> SDKII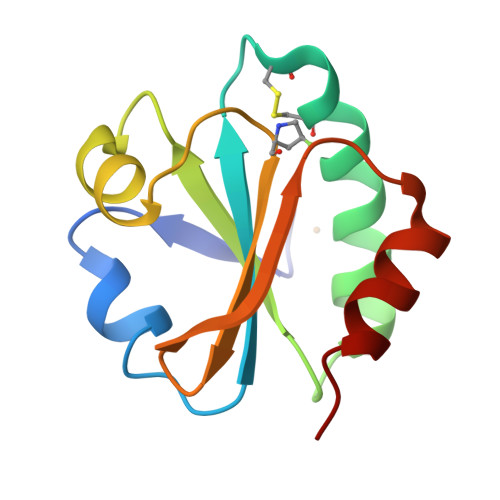HLTDDSFDTDVLKADGAILVDFWAEWCGACKMIAAILDEIADEYQGKLTVAKLNIDQNAGTAAKYGIRGIPTLLLFKNGEVAATKVGALSKGQLKEFLDANLA> GSHMRFDEFGNIITDSAVAEEPEPELPGVTEEALRLKEAALEELAAQEVTAPLVPLAVSAFLTSRKKAAAAELADWMQSPE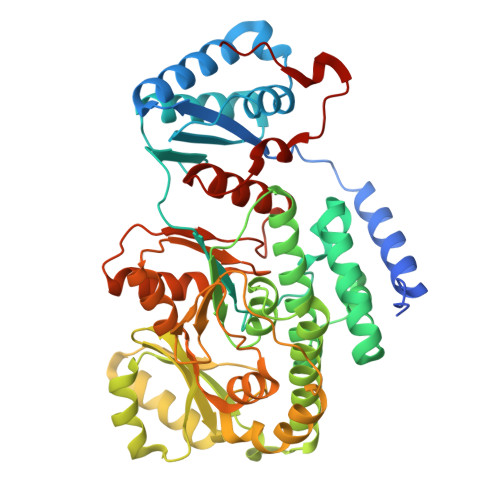GQASSLESIGRSLSRRNHGRSRAVVLAHDHDEAIKGLRAVAAGKQAPNVFSVDGPVTTGPVWVLAGFGAQHRKMGKSLYLRNEVFAAWIEKVDALVQDELGYSVLELILDDAQDYGIETTQVTIFAIQIALGELLRHHGAKPAAVIGQSLGEAASAYFAGGLSLRDATRAICSRSHLMGEGEAMLFGEYIRLMALVEYSADEIREVFSDFPDLEVCVYAAPTQTVIGGPPEQVDAILARAEAEGKFARKFATKGASHTSQMDPLLGELTAELQGIKPTSPTCGIFSTVHEGRYIKPGGEPIHDVEYWKKGLRHSVYFTHGIRNAVDSGHTTFLELAPNPVALMQVALTTADAGLHDAQLIPTLARKQDEVSSMVSTMAQLYVYGHDLDIRTLFSRASGPQDYANIPPTRF>[2x]MEQISISSPRKRIYHNILETIGGTPLVELHGVTEHPRIKKGTRILVKLEYFNPMSSVKDRVGFNIVYQAIKDGRLKPGMEIIESTSGNTGIA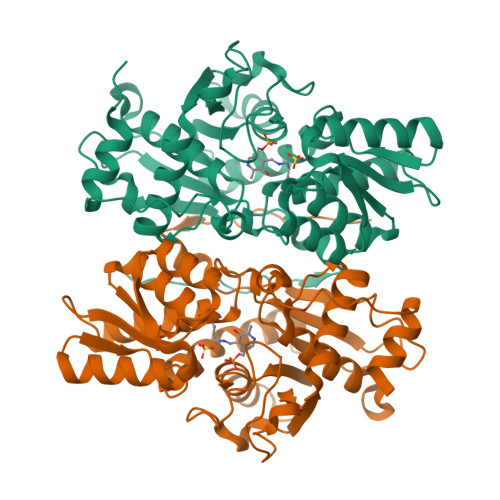LCQAGAVFGYRVNIAMPSTMSVERQMIMKAFGAELILTEGKKGMPGAIEEVNKMIKENPGKYFVANQFGNPDNTAAHHYTANEIWEDTDGEVDIVVSAVGTSGTVIGVAEKLKEKKKGIKIIAVEPEESAVLEGKAKGPHGIQGIGAGFIPDIYKKEFVDEIIPIKTQDAWKMARAVVKYDGIMCGMSSGAAILAGLKEAEKPENEGKTIVIIVPSCGERYLSTDLYKIKDEGTKIQILDSLLNEHHHHHH> MSAIKPDMKIKLRMEGNVNGHHFVIDGDGTGKPFEGKQSMDLEVKEGGPLPFAFDILTTAFAYGNRVFAKYPDNIQDYFKQSFPKGYSWERSLTFEDGGICNARNDITMEGDTFYNKVRFYGTNFPANGPVMQKKTLKWEPSTEKMYVRDGVLTGDVETALLLEGNAHYRCDFRTTYKAKEK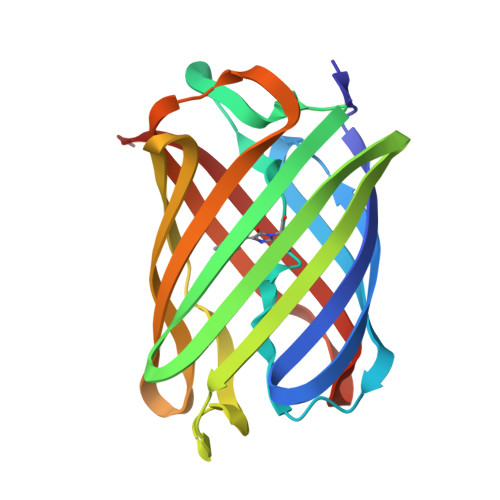GVKLPGAHFVDHCIEILSHDKDYNKVKLYEHAVAHSGLPN Artemether | C16 H26 O5 | 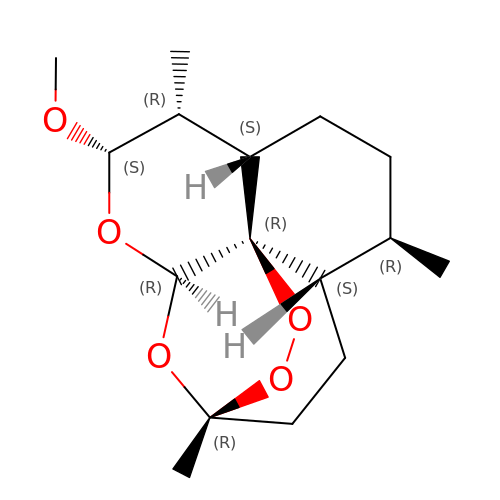SXYIRMFQILZOAM-HVNFFKDJSA-N> 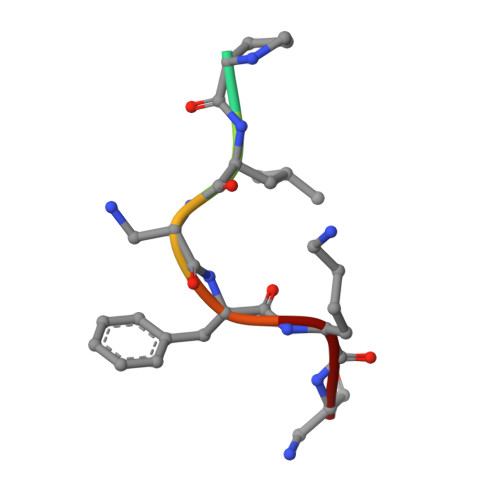KPLAFKA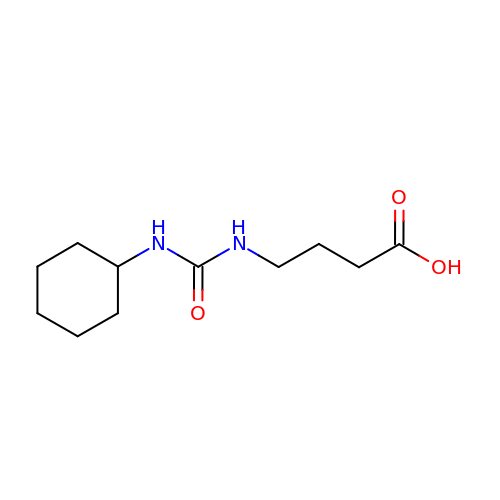4-{[(CYCLOHEXYLAMINO)CARBONYL]AMINO}BUTANOIC ACID | C11 H20 N2 O3 | WSVFRGGLURJIMG-UHFFFAOYSA-N> RPHPDHELVVCGAPDAAALTGLLTRVRAAATALSRPELTDLAAGLAAAHRGDVPARFAAAVRDADGLVAALDRALGHLAEGGRRLLDAGRGLFLVVGGPLRVGLLFPGQAAPVHADRGALGHLLGDADAGTGSDPDSGVKPAEPVDTAVAQPAIIADSLAGIRWLDRLGARPVGALGHSLGELAALSWAGALDADDTLALARARGEAMSVATEAPSGMLSLRADLAAARELAAGTGAVVAVDNGERHVVVAGTR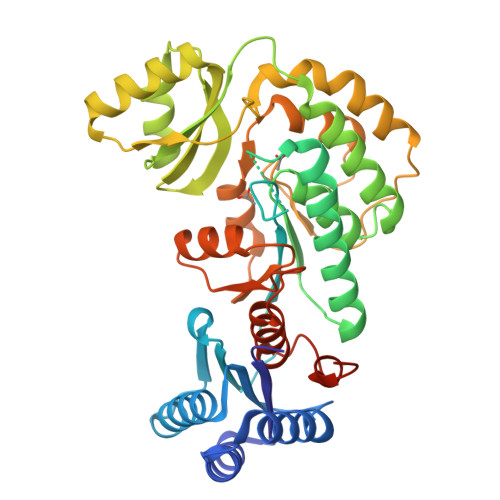PELDRVAEAARHAGIEATPLAVSHAFHSPLMAPAAEALRRAAGRLPWRRPERPVASTVTGAWWADEDPVEVLVRQLTGPVRFREALGLLDADLLVEVGPGRMLSALAEAAGRTAVSLDAGAASAAGMAAGTAALFAAGAVDDATPFFAGRFTRPFDRDREREFLVNP>[2x]KVFQWFGSNESGAEFGSQNLPGVEGKDYIWPDPNTIDTLISKGMNIFRVPFMMERLVPNSMTGSPDPNY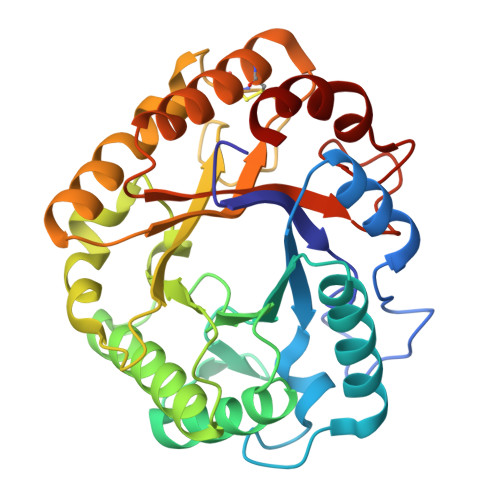LADLIATVNAITQKGAYAVVDPHNYGRYYNSIISSPSDFQTFWKTVASQFASNPLVIFDTNNEYHDMDQTLVLNLNQAAIDGIRSAGATSQYIFVEGNSWTGAWTWTNVNDNMKSLTDPSDKIIYEMHQYLDSDGSGTSATCVSSTIGQERITSATQWLRANGKKGIIGEFAGGANDVCETAITGMLDYMAQNTDVWTGAIWWAAGPWWGDYIFSMEPDNGIAYQQILPILTPYL>AGWNAYIDNLMADGTCQDAAIVGYKDSPSVWAAVPGKTFVNITPAEVGVLVGKDRSSFYVNGLTLGGQKCSVIRDSLLQDGEFSMDLRTKSTGGAPTFNVTVTKTDKTLVLLMGKEGVHGGLINKKCYEMASHLRRSQY[2x];>PPPPPPPPPPPP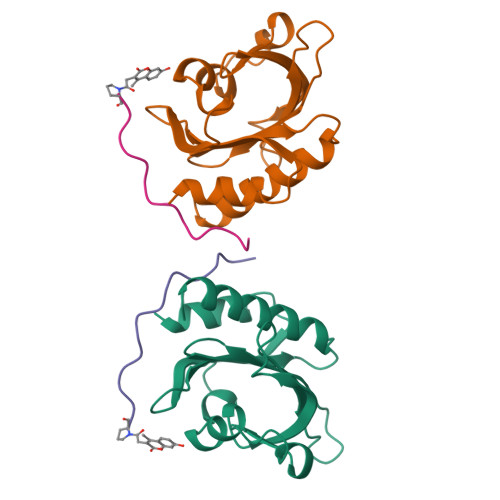PPP[2x]>[2x]SATTNPLQSIFLTPETAKACIDAAGGTPLYAYSIDKLEEAADACLAFPNAYGLTVRYAMKACPNASILKYFHSKNIHVDASSGFEVRRAM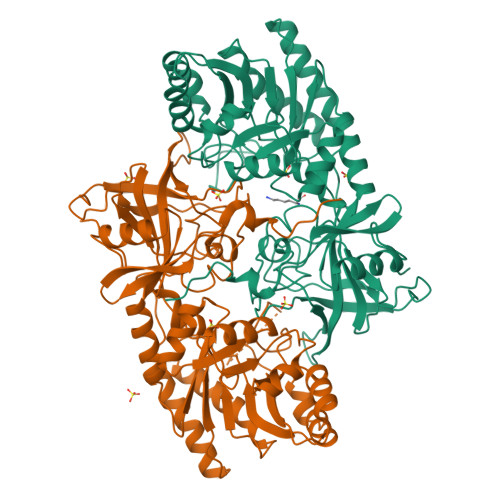DAGVPAENISLSTQELPEDFAALVDMGVKLNACSVSQLERFGEHYAGKGAKVGVRVNPGVGSGGFSASTTGFSKTNVGGPSSSFGIWHELVTDGTVPDIVERYGLEVERIHTHIGSGSDPEIWQQVATKSLSFCKVFPTVKTMNLGGGYKVGRNKGEVTTDLQKIGKPVADAFKKFAEKEGRELQMEIEPGTYLVAMAGALVSKVQDKVHTTGENSHTFLKLDAGMTDVLRPSLYGAVHPITILPGSGNSADVGDETESVVVVGHCCESGDLMTPAPGEPEQLAEQELRAAAVGDILVMDGSGAYCSGMSTKNYNSFPEAPEVLVDKAGKAHLIRKRQTLSQIYENEISVE> MADKELKFLVVDDFSTMRRIVRNLLKELGFNNVEEAEDGVDALNKLQAGGFGFIISD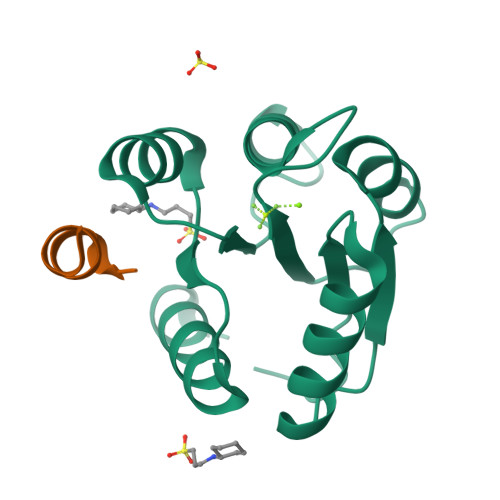WNMPNMDGLELLKTIRADSAMSALPVLMVTAEAKKENIIAAAQAGASGYVVKPFTAATLEEKLNKIFEKLGM;> ASQDQVDDLLDSLGF> GAMTFTRYSRLRVIAEIRHGDIFHSANIVSSIEFDRDDELFATAGVSRCIKVFDFSSVVNEPADMQCPIVEMSTRSKLSCLSWNKHEKNHIASSDYEGIVTVWDVTTRQSLMEYEEHEKRAWSVDFSRTEPSMLVSGSDDCKVKVWCTRQEASVINIDMKANICCVKYNPGSSNYIAVGSADHHIHYYDLRNISQPLHVFSGHKKAVSYV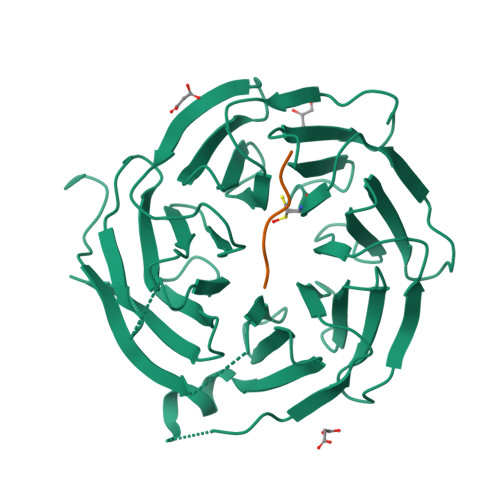KFLSNNELASASTDSTLRLWDVKDNLPVRTFRGHTNEKNFVGLTVNSEYLACGSETNEVYVYHKEITRPVTSHRFGSPDMDDAEEEAGSYFISAVCWKSDSPTMLTANSQGTIKVLVLAA;> XEHFIVPDLY>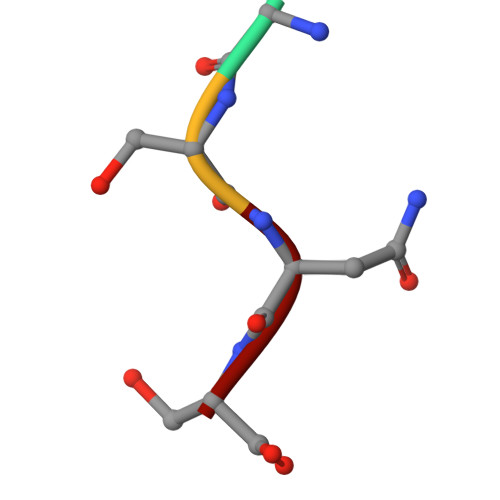 GSNS>EMANRLAGLE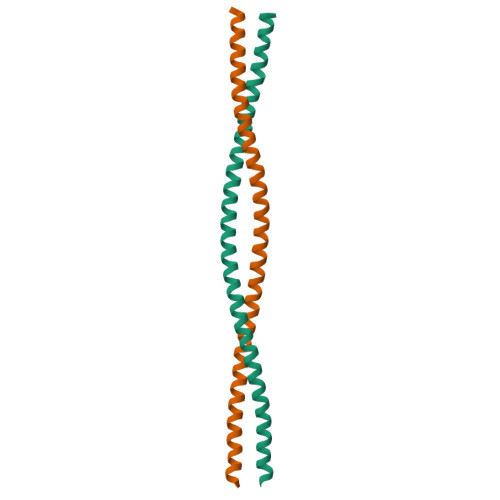NSLESEKVSREQLIKQKDQLNSLLASLESEGAEREKRLRELEAKLDETLKNLELEKLARMELEARLAKTEKDRAILELKLAEAIDEKSKLE[2x]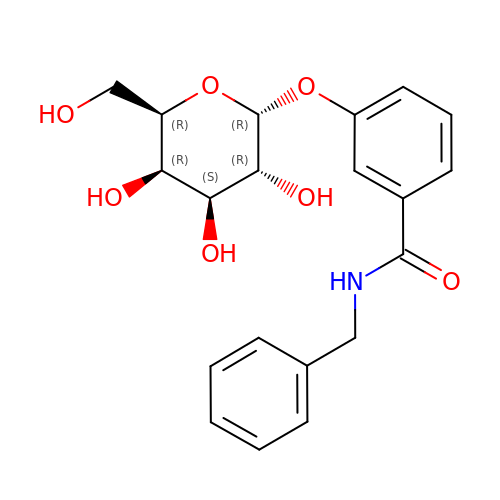N-BENZYL-3-(ALPHA-D-GALACTOS-1-YL)-BENZAMIDE | C20 H23 N O7 | FSMWGHKWKYCPKE-QTVCLEQKSA-N> MHHHHHHSSGLVPRGSLQLLEIKARGRFGCVWKAQLMNDFVAVKIFPLQDKQSWQSEREIFSTPGMKHENLLQFIAAEKRGSNLEVELWLITAFHDKGSLTDYLKGNIITWNELCHVAET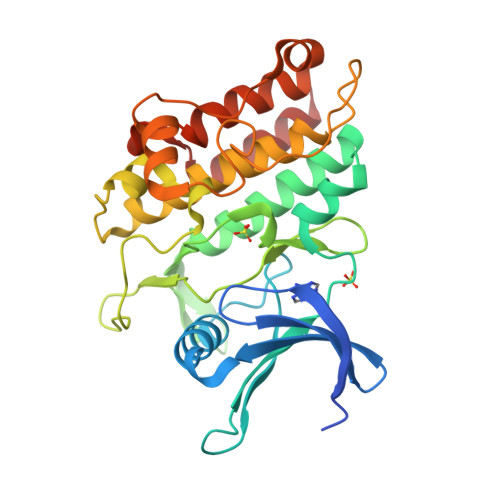MSRGLSYLHEDVPWCRGEGHKPSIAHRDFKSKNVLLKSDLTAVLADFGLAVRFEPGKPPGDTHGQVGTRRYMAPEVLEGAINFQRDAFLRIDMYAMGLVLWELVSRCKAADGPVDEYMLPFEEEIGQHPSLEELQEVVVHKKMRPTIKDHWLKHPGLAQLCVTIEECWDHDAEARLSAGCVEERVSLIRRSVNG cAMP response element binding Protein 3 (CREB3) is an endoplasmic reticulum (ER) membrane‐bound transcription factor, which belongs to the basic leucine zipper (bZIP) superfamily of eukaryotic transcription factors. CREB3 plays a role in the ER‐stress induced unfolded protein response (UPR) and is a multifunctional cellular factor implicated in a number of biological processes including cell proliferation and migration, tumor suppression, and immune‐related gene expression.

To gain structural insights into the transcription factor, we determined the crystal structure of the conserved bZIP domain of chicken CREB3 (chCREB3) to a resolution of 3.95 Å. The X‐ray structure provides evidence that chCREB3 can form a stable homodimer. The chCREB3 bZIP has a structured, pre‐formed DNA binding region, even in the absence of DNA, a feature that could potentially enhance both the DNA binding specificity and affinity of chCREB3. Significantly, the homodimeric bZIP possesses an intermolecular disulfide bond that connects equivalent cysteine residues of the parallel helices in the leucine zipper region. This disulfide bond in the hydrophobic core of the bZIP may increase the stability of the homodimer under oxidizing conditions. Moreover, sequence alignment of bZIP sequences from chicken, human, and mouse reveals that only members of the CREB3 subfamily contain this cysteine residue, indicating that it could act as a redox‐sensor. Taken together, these results suggest that the activity of these transcription factors may be redox‐regulated and they may be activated in response to oxidative stress.

>[7x]MAGPEPLAALPDGDLLDFLLNDDAPAAGSPAGDGPLLGDWVLPELELLDKEMDSFISSLLSPSEDEPCLLQGCLPADSDSSTSEDQNPFHSSGSDVASSPQSSDIVQFDHNYSLHQDWPALESVRSDMAEGDVSIDLETWMCLEGTNETLQESCSFPVTVAVDAGPQLMPGAPMQSNFPELVLTEEERQLLEKDGVSLPTCLPLTKAEERLLKKVRRKIRNKQSAQDSRRRKKIYVDGLENRVAACTAQNHELQKKVQLLQKQNMSLLEQLRKLQALVRQSTTKTTTASTCIMVLVLSFCLILSPSLYSFGSRGPQPEFRVLSRQIREFPNKVWQAAPAVQEEVVLERLSPEPEDTSLGSLNQSREEGQSPPKPDPRSAFNGNSSSDPPAGSELGHPQPQEQQSRRDALHSEVLAPWKDENQEWVERTTSVVIQQHRTDEM Breakdown is then initiated with the conversion of the C‐3 hydroxyl group to a ketone (cholest‐4‐en‐3‐one, cholestenone) by the oxidase ChoD, and further oxidation at the C‐26 “tail” region via a three‐step process involving oxidation to the hydroxyl, aldehyde, and carboxylic acid species. These sidechain‐modifying reactions are catalysed by the cytochromes P450 CYP125A1 and CYP142A1 (CYP125 and CYP142 hereafter). Comparison of the effect of complementing a CYP125 knockout in the CDC1551 strain of Mtb (which does not express the CYP142 protein), with CYP125 or CYP142 reveals that the two enzymes are functionally redundant with respect to growth on cholesterol. Here we present a series of compounds based on an ethyl 5‐(pyridin‐4‐yl)‐1H‐indole‐2‐carboxylate pharmacophore which bind strongly to both Mtb cholesterol oxidases CYP125 and CYP142.

The replacement of the cyclohexyl group with a piperazine ring, 14, showed a significant drop in affinity. In the X‐ray co‐crystal structures of compounds 14 and 15 in complex with CYP125, the pyridine coordinates directly with the heme iron, but in an orientation that is rotated almost exactly 180° around the heme vertical axis relative to compound 4.

>[3x]NGPSPNLPPGFDFTDPAIYAERLPVAEFAELRSAAPIWWNGQDPGKGGGFHDGGFWAITKLNDVKEISRHSDVFSSYENGVIPRFKNDIAREDIEVQRFVMLNMDAPHHTRLRKIISRGFTPRAVGRLHDELQERAQKIAAEAAAAGSGDFVEQVSCELPLQAIAGLLGVPQEDRGKLFHWSNEMTGNEDPEYAHIDPKASSAELIGYAMKMAEEKAKNPADDIVTQLIQADIDGEKLSDDEFGFFVVMLAVAGNETTRNSITQGMMAFAEHPDQWELYKKVRPETAADEIVRWATPVTAFQRTALRDYELSGVQIKKGQRVVMFYRSANFDEEVFQDPFTFNILRNPNPHVGFGGTGAHYCIGANLARMTINLIFNAVADHMPDLKPISAPERLRSGWLNGIKHWQVDYTGRCPVAH> GHMATGTRYAGKVVVVTGGGRGIGAGIVRAFVNSGA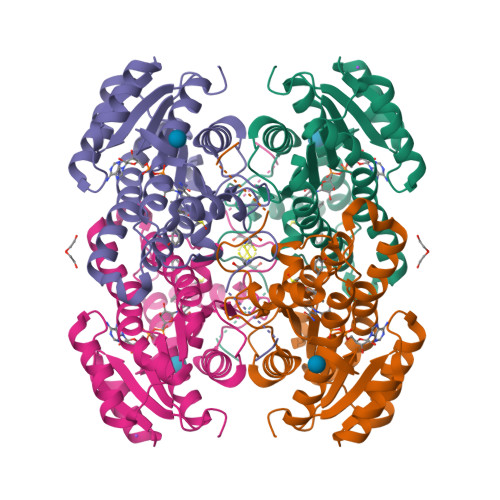RVVICDKDESGGRALEQELPGAVFILCDVTQEDDVKTLVSETIRRFGRLDCVVNNAGHHPPPQRPEETSAQGFRQLLELNLLGTYTLTKLALPYLRKSQGNVINISSLVGAIGQAQAVPYVATKGAVTAMTKALALDESPYGVRVNCISPGNIWTPLWEELAALMPDPRATIREGMLAQPLGRMGQPAEVGAAAVFLASEANFCTGIELLVTGGAELGYGCKASRSTPVDAPDIPSGS>MSDENYRDIALAFLDESADSGTINAWVNEFAYQGFDPKRIVQLVKERGTAKGRDWKKDVKMMIVLNLVRGNKPEAMMKKMSEKGASIVANLISVYQLKEGNPGRDTITLSRVSAAFVPWTVQALRVLSESLPVSGTTMDAIAGVTYPRAMMHPSFAGIIDLDLPNGAGATIADAHGLFMIEFSKTINPSLRTKQANEVAATFEKPNMAAMSGRFFTREDKKKLLIAVGIIDEDLVLASAVVRSAEKYRAKVGK[11x];> MSDENYRDIALAFLDESADSGTINAWVNEFAYQGFDPKRIIQLVKERGTAKGRDWKKDVKMMIVLNLVRGNKPEAMMKKMSEKGASIVANLISVYQLKEGNPGRDTITLSRVSAAFVPWTVQALRVLSESLPVSGTTMDAIAGVTYPRAMMHPSFAGIIDLDLPNGAGATIADAHGLFMIEFSKTINPSLRTKQANEVAATFEKPNMAAMSGRFFTREDKKKLLIAVGIIDEDLVLASAVVRSAEKYRAKVGK

Toscana virus is an enveloped negative-strand ribonucleic acid (RNA) virus that belongs to the genus phlebovirus in the Bunyaviridae family. The genome of phleboviruses, like other bunyaviruses, is tightly packed with N into ribonucleoprotein complexes (RNPs). In this study, we have elucidated structures of the hexameric RNA-free (apo) N and of hexameric N in complex with a single-stranded nonameric RNA. As in the RVFV N structure, each N monomer consisted of a core domain comprised of two α-helical lobes (the upper and the lower lobe), and an amino-terminal α-helical arm which was divided by a short linker, hinge II, in α1 and α2.

Using an unfolding/refolding protocol, nucleic acid-free N was obtained, as judged from the A260/A280 ratio of 0.6. The apo structure contained 12 molecules of N in the asymmetric unit, which were organized in two hexameric rings. In the hexameric rings of the apo structure, an almost perfect six-fold symmetry between the six monomers was observed. Oligomerization was driven by the amino-terminal arm, which bound into a hydrophobic groove of the neighboring monomer at the outside of the hexamer (pockets I and II in Figure 1E and F). The interaction of helix α1 with the neighboring monomer included hydrogen bonds and hydrophobic contacts, and a salt bridge between Lys83 and Glu29 of the opposing monomer. In the apo N structure, Tyr32 from hinge I, Lys204 from the lower lobe and Lys79 from the upper lobe of the adjacent subunit are in close proximity to each other and cap the RNA-binding tunnel. In the absence of RNA, Tyr32, Lys204 and Lys79 localize closely together in the RNA-binding tunnel. Furthermore, it can be envisaged that the proposed inter-subunit shift is energetically not favoured over the planar architecture, since we do not observe it in the apo N hexamer.>[2x]MGITAPTPLTSEHNLADFCCSDHGMNEWLKKKALKNHSSGLSRVYVICIANTRQVIGYYCLSTGSIQRNLAPGAMRRNAPESLPVVVLGRLAIDQAWAGKGLGVALLKDAVYRTMSIAQQVGVRALIVHALDDSVRNFYLKYAFVPSPFQSL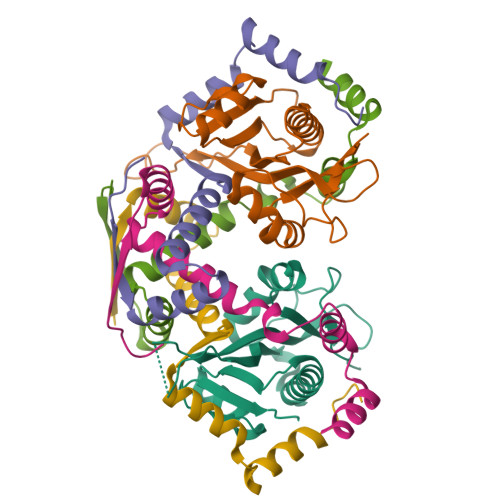TLLYPITLELEHHHHHH;>MKPESKEAPINIRAKASQRDLIDMAANLVAKSRTDFMLDAACREAQDILLDQRLFILDDEQYDAFLAALDAPITAERQAKINALMNRKSPWE[4x]>GMSQNRQLLYPREEMVSLVRSLDR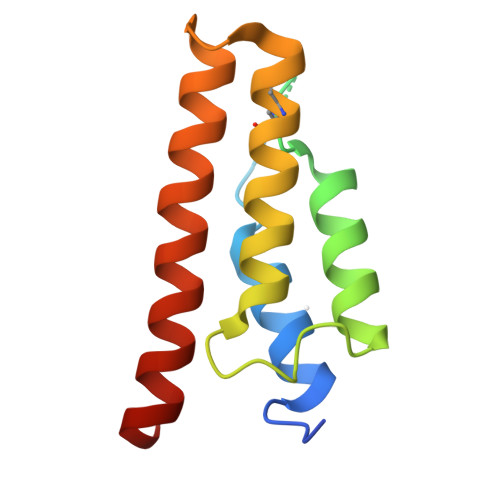PQENGLFSQDVLLQYPELAESYTKVCPNRCDLATAADRAAKGAYGYDVQLTTLKEDIRLMVNNCILFNGAEGAYADAARTFEKFAMGKIDAYISQKVGGRRL[2x]> GSMASEIHMTGPMCLIENTNGRLMANPEALKILSAITQPMVVVAIVGLYRTGKSYLMNKLAGKKKGFSLGSTVQSHTKGIWMWCVPHPKKPGHILVLLDTEGLGDVEKGDNQNDSWIFALAVLLSSTFVYNSIGTINQQAMDQLYYVTELTHRIRSKSSPDENENEVEDSADFVSFFPDFVWTLRDFSLDLEADGQPLTPDEYLTYSLKLKKGTSQKDETFNLPRLCIRKFFPKKKCFVFDRPVHRRKLAQLEKLQDEELDPEFVQQVADFCSYIFSNSKTKTLSGGIQVNGPRLESLVLTYVNAISSGDLPCMENAVLALAQIENSAAVQKAIAHYEQQMGQKVQLPTETLQELLDLHRDSEREAIEVFIRSSFKDVDHLFQKELAAQLEKKRDDFCKQNQEASSDRCSALLQVIFSPLEEEVKAGIYSKPGGYRLFVQKLQDLKKKYYEEPRKGIQAEEILQTYLKSKESMTDAILQTDQTLTEKEKEIEVERVKAESAQASAKMLQEMQRKNEQMMEQKERSYQEHLKQLTEKMENDRVQLLKEQERTLALKLQEQEQLLKEGFQKESRIMKNEIQDLQTKMRRRKACTIS

The guanylate-binding proteins (GBPs) play critical roles in cell-autonomous immunity against a diverse range of bacterial, viral, and protozoan pathogens. GBP1 contains an N-terminal large GTPase (LG) domain and a C-terminal helical region, which can be further divided into a middle domain (MD) that contains the α7-α11 helices and a GTPase effector domain (GED) that consists of the α12-α13 helices. The GED folds back and interacts with LG and MD, which is important to maintain GBP1 at the resting state. Recent studies have discovered that IpaH9.8 ubiquitinates and degrades a subset of GBPs, which is important for S. flexneri to suppress host defense and replicate in the cells.

GBP1 is farnesylated at Cys589, and this modification is important for its localization to the Golgi apparatus and recruitment by various pathogens. We subsequently determined the crystal structure of GBP1F. Interpretable electron density is present for the farnesyl group, as well as the entire C-terminal tail of GBP1. The farnesyl group is accommodated in a pocket formed by His378, Gln381, Lys382, Ala385 from the α9 helix and Tyr524, His527, Leu528, Leu531 from the α12 helix. These interactions pull the α12 helix towards the α9 helix, and cause the GED domain to become more tightly fastened to the rest of the protein. In this conformation, the α7 helix remains bent; while the N-terminal half the α12 helix, as well as the majority of the MD domain, undergoes a ~10° rotation when compared to the previously determined full-length GBP1 structure. In a way, the GBP1F structure likely reflects GBP1 at its most tense state. By creating additional interactions between the GED domain and the MD domain, the farnesyl group appears to function as the second tier of bolt to lock the GED domain to the rest of the protein. A bending of the α7 helix is forced in this conformation.> MDGSGEQPRGGGPTSSEQIMKTGALLLQGFIQDRAGRMGGEAPELALDPVPQDASTKKLSESLKRIGDELDS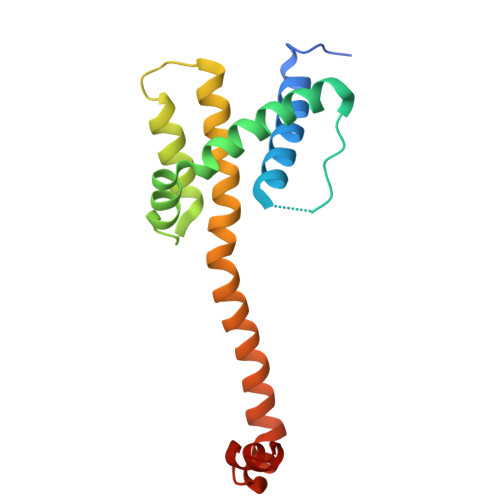NMELQRMIAAVDTDSPREVFFRVAADMFSDGNFNWGRVVALFYFASKLVLKALSTKVPELIRTIMGWTLDFLRERLLGWIQDQGGWDGLLSYFGSS>MSSLLVKKLVESATTPMRGSEGAAGYDISSVEDVVVPAMGRIAVS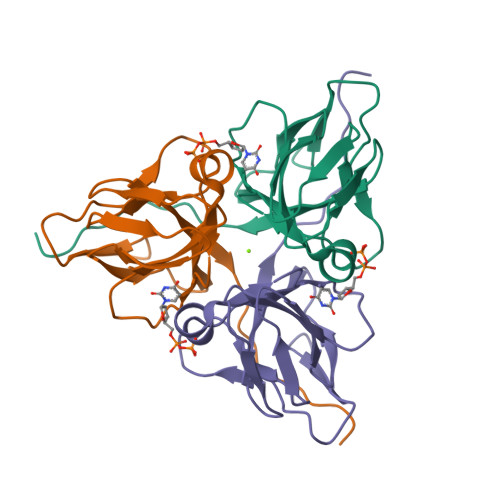TGISIRVPDGTYGRIAPRSGLAYKYGIDVLAGVIDEDYTGEVKVILYNTTERDYIIKKGDRIAQLILEQIVTPGVAVVLDLSDTARGSGGFGSTGI[2x]>MAAFSKYLTARNSSLAGAAFLLLCLLHKRRRALGLHGKKSGKPPLQNNEKEGKKERAVVDKVF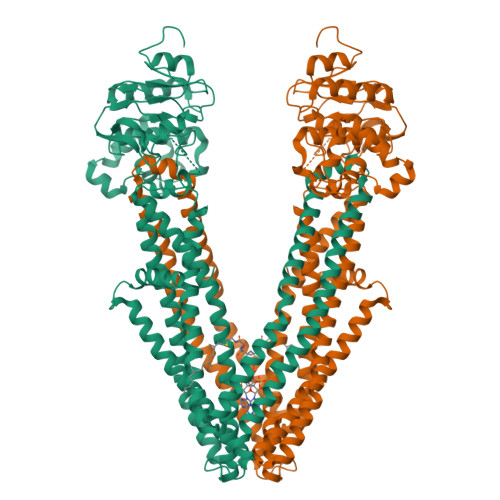FSRLIQILKIMVPRTFCKETGYLVLIAVMLVSRTYCDVWMIQNGTLIESGIIGRSRKDFKRYLLNFIAAMPLISLVNNFLKYGLNELKLCFRVRLTKYLYEEYLQAFTYYKMGNLDNRIANPDQLLTQDVEKFCNSVVDLYSNLSKPFLDIVLYIFKLTSAIGAQGPASMMAYLVVSGLFLTRLRRPIGKMTITEQKYEGEYRYVNSRLITNSEEIAFYNGNKREKQTVHSVFRKLVEHLHNFILFRFSMGFIDSIIAKYLATVVGYLVVSRPFLDLSHPRHLKSTHSELLEDYYQSGRMLLRMSQALGRIVLAGREMTRLAGFTARITELMQVLKDLNHGKYERTMVSQQEKGIEGVQVIPLIPGAGEIIIADNIIKFDHVPLATPNGDVLIRDLNFEVRSGANVLICGPNGCGKSSLFRVLGELWPLFGGRLTKPERGKLFYVPQRPYMTLGTLRDQVIYPDGREDQKRKGISDLVLKEYLDNVQLGHILEREGGWDSVQDWMDVLSGGEKQRMAMARLFYHKPQFAILDECTSAVSVDVEGYIYSHCRKVGITLFTVSHRKSLWKHHEYYLHMDGRGNYEFKQITEDTVEFGSGSGLVPRGSGGGGSGGGGSGGHHHHHHHH[2x]4-chloro-3-[1-(2-chloro-6-fluorobenzoyl)-1,2,3,4-tetrahydroquinolin-6-yl]-N-methylbenzamide | C24 H19 Cl2 F N2 O2 | 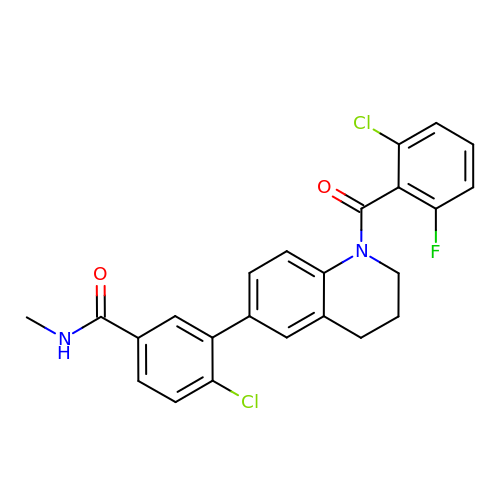NWECRSKQCPBSPW-UHFFFAOYSA-N>[22x]MAQVINTNSLSLLTQNNLNKSQSALGTAIERLSSGLRINSAKDDAAGQAIANRFTANIKGLTQASRNANDGISIAQTTEGALNEINNNLQRVRELAVQSANSTNSQSDLDSIQAEITQRLNEIDRVSGQTQFNGVKVLAQDNTLTIQVGANDGETIDIDLKQINSQTLGLDSLNVQKAYDVKDTAVTTKAYANNGTTLDVSGLDDAAIKAATGGTNGTASVTGGAVKFDADNNKYFVTIGGFTGADAAKNGDYEVNVATDGTVTLAAGATKTTMPAGATTKTEVQELKDTP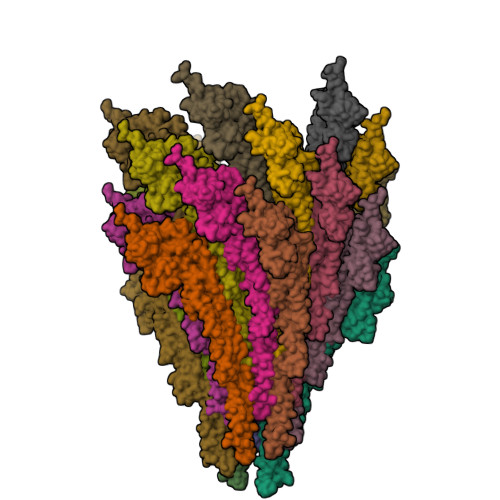AVVSADAKNALIAGGVDATDANGAELVKMSYTDKNGKTIEGGYALKAGDKYYAADYDEATGAIKAKTTSYTAADGTTKTAANQLGGVDGKTEVVTIDGKTYNASKAAGHDFKAQPELAEAAAKTTENPLQKIDAALAQVDALRSDLGAVQNRFNSAITNLGNTVNNLSEVRSRIEDSDYATEVSNMSRAQILQQAGTSVLAQANQVPQNVLSLLR> GGWHDE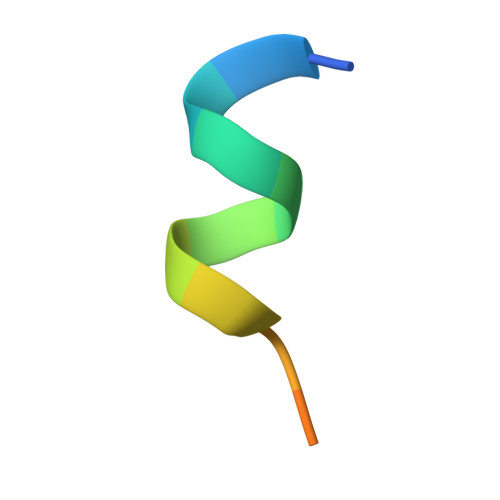ATWKPGLY>MKKHGILNSHLAKILADLGHTDKIVIADAGLPVPDGVLKIDLSLKPGLPAFQDTAAVLAEEMAVEKV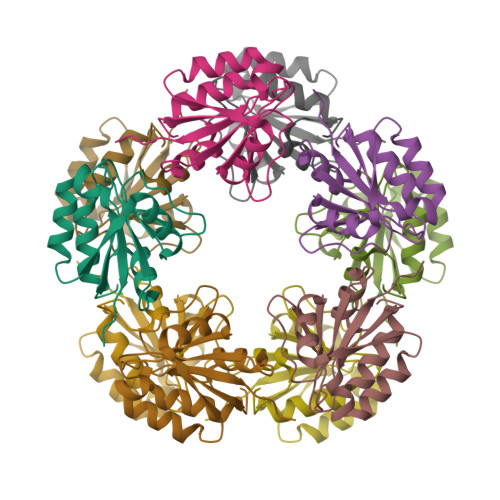IAAAEIKASNQENAKFLENLFSEQEIEYLSHEEFKLLTKDAKAVIRTGEFTPYANCILQAGVLF[5x]> MPFYDSRPPEGWPKGSINDMDYPLLGSICAVCCVFVAGSGIWMLYRLDLGMGYSCKPYKSGRAPEVNSLSGIICLLCGTMYAAKSFDFFDGGGTPFSLNWYWYLDYVFTCPLLILDFAFTLDLPHKIRYFFAVFLTLWCGVAAFVTPSAYRFAYYALGCCWFTPFALSLMRHVKERYLVYPPKCQRWLFWACVIFFGFWPMFPILFIFSWLGTGHISQQAFYIIHAFLDLTCKSIFGILMTVFRLELEEHTEVQGLPLNEPETLS

Kalium channelrhodopsin 1 from Hyphochytrium catenoides (HcKCR1) is a light-gated channel used for optogenetic silencing of mammalian neurons. The genome of H. catenoides also encodes a highly homologous cation channelrhodopsin (HcCCR), a Na+ channel with >100-fold larger Na+ to K+ permeability ratio. Here, we use cryo-electron microscopy to determine atomic structures of these two channels embedded in peptidiscs to elucidate structural foundations of their dramatically different cation selectivity. Together with structure-guided mutagenesis, we show that K+ versus Na+ selectivity is determined at two distinct sites on the putative ion conduction pathway: in a patch of critical residues in the intracellular segment (Leu69/Phe69, Ile73/Ser73 and Asp116) and within a cluster of aromatic residues in the extracellular segment (primarily, Trp102 and Tyr222).

In that regard, HcKCR1 is of particular interest as a highly efficient tool for optical neuronal silencing. The central pore between the three HcKCR1 protomers is filled with six phospholipids, which we modeled as dioleoylphosphatidylethanolamine (DOPE), three in each leaflet of the bilayer, that prevent ions from translocating through the pore. In addition, the membrane-facing outer surface of the HcKCR1 trimer is decorated with nine sterol lipids and nine phospholipids, which we modeled as DOPE molecules, although in some cases the density did not clearly exclude choline headgroups and different hydrocarbon chains. Although Asp116 is conserved in HcKCR1 and HcCCR, its mutagenetic neutralization in HcKCR1 results in conversion of the K+-selective channel into a Na+-selective one with a much smaller conductance. In the HcKCR1 structure, the presence of Ile73 and Leu69 on the helical interface between TM2 and 3 moves TM2 away by 1.4 Å (measured at the Cα atom of Val66). This helical movement slightly enlarges the vestibule, which may help accommodate a large K+ ion in the vicinity. In HcKCR1 Tyr222 forms H-bonds to Trp102 and Gln218. As a result, the extracellular channel opening is interrupted with the bulky aromatic Tyr side chain in HcKCR1 but continues deeper into the molecule in HcCCR, creating a key determinant for K+ selectivity. In HcKCR1, the Y222W mutation caused a stronger Vrev shift to more depolarized values indicating a decrease in PK/PNa than that caused by the W102Y mutation, which suggests that the residue in the position 222 is more important for K+ selectivity than that in the position 102. When the channel opens under illumination, Tyr222 (likely assisted by Phe221 and His225 on the other side of the putative conduction cation pathway) allows K+ passage but functions as a barrier to the flux of larger hydrated cations like Na+ and divalent cations.>[6x]MRPEVEQELAHTLLVELLAYQFASPVRWIETQDVFLAEQMAERIVEIGPADTLSVMAKRTLASKYEAYDAAKSAQRQILCYSKDAKEIYYDVDPIEEEPEPAPAQAATPTAPAAPAATPAAAPAPVAAPPPPGVGPAAQVPDAPVTALEIVRALIAQKLKKPYQEVPLSKAIKDLVGGKSTLQNEILGDLGKEFGSTPEKPEDTPLDELGAAMQATFDGNLGKTSQGLIARLISSKMPGGFNITTARKYLETRWGLGPGRQDGVLLLAITMEPPSRLGSEADAKAFLDDVSQKYAANAGISLSTAAAAGPAAGAGGGMLMDPAALEALTSDQKALFKQQLELIARYLKLDIRAGDKAYQASQESAKVLQSQLDLWLAEHGDFYASGIEPVFSPLKARVYDSSWNWARQDALSMYYDIIFGRLKTVDREIVSQCIRIMNRANPTLLEFMQYHIDNCPTDRGETYQLAKELGAQLIENCKEVLNANPVYKDVAIPTGPKTTIDARGNLKYEEVPRPSCRKLEHYVQQMAAGGKISEYGNRIKVQNDLAKIYKLIKQQHKLPKTSQLEIKALYSDIIRALQMNENQILGQTNGKSLGLPKKGKPKAKTETIPFLHLRKKSVMGWEYNKKLTSLYLDCLEKAARDGLTFAGKYALMTGAGAGSIGAEVLQGLISGGAHVIVTTSRYSREVTEYYQSMYSRYGARGSQLVVVPFNQGSVQDVNALVEYIYDTKNGLGWDLDYIVPFAAISEQGRQIDGIDSKSELAHRIMLTNLIRLLGAVKTQKASRGYETRPAQVILPLSPNHGTFGSDGLYSESKLGLETLFNRWESENWSNYLTICGAIIGWTRGTGLMSGNNIVAEAVEKFGVRTFSQQEMAFNLLGLMAPTIVDLCQNEPVCADLNGGLQFIPNLNELMTRERKNLTETSEIRQAVTKETAAENKVVNGEASEALYKKKIIERRANIKFDFPPLPDWKKDIQPLNDKLKGMVDLEKVIVVTGFAEVGPWGNSRTRWEMEAYGEFSLEGCIEMAWIMGLIKNYNGLIKGKPYSGWVDAKTGEPVDDKDVKPKYEKYILEHSGIRLIEPELFGGYDPNKKQLLHEVVIQEDLDPFQCSAETAEQFKREHGDKVEIFEIPESGEYTVRFKKGATLWIPKALRFDRLVAGQIPTGWDAKRYGIPDDIIQQVDPVCLFVLVSTVEALLSSGITDPYEFYKYVHVSELGNCIGSGMGGATALRGMHRDRFLDKPLQNDILQESFINTMSAWVNMLLLSSSGPIKTPVAACATAVESVDVGVETILEGKARICLVGGFDDFGEEGSYEFANMKATSNAVDEFAHGRTPQEMSRPTTTTRNGFMESQGSGVQVIMTAKLALEMGVPIYGILALTTTASDKIGRSVPAPGQGVLTTAREHRGKFPSPLLDINYRRRQIERRTKQVMEEKEAEFEYLAAEIEALKAEGRPQSEIEEYAAHRAAHIEKTAEKQAKEILRSFGNFFWKNDPTIAPLRGALAVWGLTIDDLDVASFHGTSTKANDKNESSVICQQLAHLGRKKGNAVLGIFQKYLTGHPKGAAGAWMLNGCLQVLNTGLVPGNRNADNVDKVMEQFDYIVYPNRSIQTDGIKAFSVTSFGFGQKGAQCIGVHPKYLYATLDEQTYNEYCTKVQARQKKAYRYFHNGLINNTLFQAKEKAPYTDEQLSAVLLNPDARVVEDKKTGQLIFPPNFMKLSEKTQAAAQPKVSLESVLSREARRLESVNTRVGVDVEDISAINTDNDTFLDRNFTEAEQKYCLASKSGRSPQKAFAGRWTAKEAVFKALGVSSKGAGAALKDIEILVDENGAPTVSLHGAAAEAAKKAGIKSVSVSISYTDSQAAAIATAQL;>MY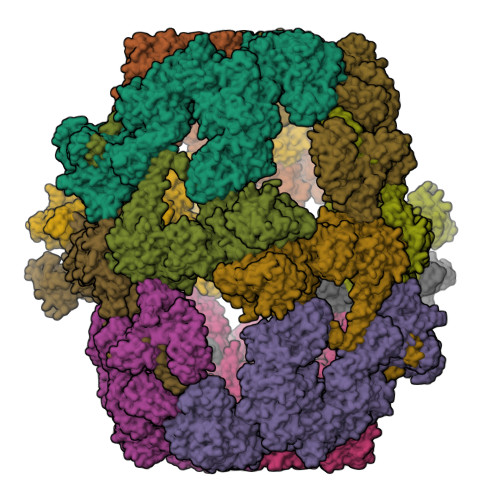GTGTGPQTGAVTPRSSASLRPLTLSHGSLETSFLIPTGLHFHASRLKDEFIASLPPPTDELAQDDEPSSVPELVARYMGYIANQVAEGEDDAQGSYEEVLKLILNEFERAFLQGNDVHALVATLPGIDAKKLEVIRSYFAARAATNRAMRAHQSALLRAAEEGEARIYSIFGGQGNIEEYFEELRELYKTYPSFVGHLIVSSAELLQILASHPSAEKLYSKGLDIMHWLHNPDATPDTDYLISAPVSFPLIGLVQLAHYQVTCKVQGLHPGILRDRISGTTGHSQGIVLAAVTAAADSWESFEDLAKSALTILFWIGARSQQTFPRTSMSPSLLQEAIDNGEGTPTPMLSIRDLPQAEVQKHIDQTNQYLPEDQHISISLINSPRNLVVSGPPRSLCGLNAQLRKVKAPTGLDQARIPYSERKIRFVNRFLPITAPFHSKYLAGAAELIAEDLKDISIEVERLGIPVYDTNTGEDIRQTVTGNVVPALIRMITNDPVHWEKATVFPEATHILDFGPGGISGLGVLTSRNKDGTGVRVILAGTVNGTVAEVGYKSELFDRDEEHAVKYAVDWVKEYGPRLIKTSSGRIYVDTKMSRLLGLPPLMVAGMTPTTVPWDFVAATMNAGYQIELAGGGYFNAKMMTEAISKIERAIPPGRGITVNLIYVNPHAMAWQIPLLGRLRAEGVPIEGLTIGAGVPSIEVANEYIQTLGLKHISFKPGSVDAIQAVINIAKANPTFPVILQWTGGRGGGHHSYEDFHAPILAMYSRIRRQENIILVAGSGFGGAEDTYPYLTGAWSTKYGYPPMPFDGCLFGSRMMVAKEAHTSPEAKQAIVDAPGLDDSEWEKTYKGPAGGVITVRSEMGEPIHKLATRGVLFWAEMDQKIFSLPKEKRVAELKKNRDYIIRKLNADFQKVWFGKNKKGEVVDLEDMTYGEVVRRMVELLYVKDEKRWIDHSFAKLTADFIHRVEERFTTAASQPSLIQSYSDLDEPYSAVERVLAHYPEAETQLISAQDVQHFLLLCKRRGQKPVTFVPALDEDFEFYFKKDSLWQSEDLAAVIDRDVGRTCILQGPMAAKHSTKVDEPIKEILDGIHNGHIAALKRDLYDNDESKIPTIEYFGGKLKDPEVQLDFEGVTISYDVHKNTYRVSNNPSVPLPPLDAWLSALAGPNRTWRYALLQSEVIVQGHKYQTNPMKKIFAPARGLFVEIQYPNDPAKTVITVKEQPRPNRYIDVIEAKLVGDKEIVVNLIKDTNALGEPVALPLRFTYRPEAGYAPIHEIMEGRNDRIKEFYWRCWFGQDPLDLDAPVTSKFDGGEAVITSEAINEFVHAVGNTGEAFVDRPGKTMYAPMDFAIVVGWKAITKPIFPRTIDGDLLKLVHLSNQFRMFPGAEPLKKGDKVYTTAQVNAVINQESGKMVEVCGTITRDGKPVMEVISQFLYRGVYTDYENTFQRKVETPMQVHLATTKDIAILRSKQWFVLDDVATPEEFLLGKTLTFRLHTLVHFKNRNVYSHVETRGQVLVELPTKEIIQVATVEYVAGESHGNPVIDYLQRNGQSIEQPVNFENPIPLGGKAPLQLRAPASNETYARVSGDYNPIHVSRVFAAYANLPGTITHGMYSSAAVRSLVETWAAENKIGRVRSFHASLTGMVLPNDDINVKLQHVGMVGGRKIIKVEATNKETEEKVLLGEAEIEQPVTAYVFTGQGSQEQGMGMDLYANSPVAREVWDRADKYLRDTYGFAITDIVRNNPKELTIHFGGPLGKKIRANYMAMTFETVAADGSIKSERIFKDIDENTTSYTFRSPNGLLSATQFTQPALTLMEKASFEDMKAKGLVPRDSTFAGHSLGEYSALAALADVMPIESLVSVVFYRGLTMQVAVERDATGRSNYGMCAVNPSRISKTFNEEALRFVVGAVAETTGWLLEIVNYNIANMQYVCAGDLRALDTLTSVTNFIKAMKIDIEQMRREYSPDKVKEELVEIIKKCAAETEAKPKPLELQRGFATIPLRGIDVPFHSTFLRSGVKPFRNFLLKKINKTSIDPAKLIGKYIPNVTAKPFALTKEYFEDVYRLTNSPRIAHVLANWEKYQDDNSTLSASVANTSSETNGVNGVNGAVDVNGQNGVNGVNGH[6x]Here we describe extendable linear, curved and angled protein building blocks, as well as inter-block interactions, that conform to specified geometric standards; assemblies designed using these blocks inherit their extendability and regular interaction surfaces, enabling them to be expanded or contracted by varying the number of modules, and reinforced with secondary struts. We construct twistless helix repeat (THR) protein blocks from identical straight α-helices (typically 2–4 helices in each unit); the length of the blocks can be varied simply by varying the number of repeat units. Restricting helical geometry to ideal straight helices with zero helical twist in principle considerably limits what types of structure could be built, but this is more than compensated by the great simplification of downstream material design, as illustrated below. Using X-ray crystallography and electron microscopy, we validate nanomaterial designs ranging from simple polygonal and circular oligomers that can be concentrically nested, up to large polyhedral nanocages and unbounded straight ‘train track’ assemblies with reconfigurable sizes and geometries that can be readily blueprinted.

To generate expandable nanocages, flat cyclic components that form the faces of the cages were linked through noncovalent handshake interactions at the specified angle. For the flat cyclic component, we used a ring design with 12 repeats (R12B) constructed from curve units, and split the 12 repeats into either 3 subunits with 4 repeats each (C3) or 4 subunits with 3 repeats each (C4), depending on the desired polyhedral symmetry architecture. We then fused linear THR arms onto each subunit constrained to point outward parallel to a radial vector emanating from the symmetry axis, but offset such that when the C2 interface is formed, the C2 axis is along a radial vector. For tetrahedra (T3), octahedra (O3) and icosahedra (I3) built from flat C3-symmetric objects, the out-of-plane handshake angles that are needed to join the flat objects are 70.5°, 109.5° and 138.2°, respectively. Tetrahedral, octahedral ‘cubic’ and icosahedral structures with C3 rings at respective axes (T3, O3 and I3), and octahedral structures with C4 rings at the respective axes (O4) were constructed by incorporation of the appropriate C2 interface. Designed geometric features including the spindle-like twofold handshake interface and the flat ‘in-plane’ ring areas with distinct holes are clearly evident.

>MEELREIAERAEADMREISELAEELVEDPVYAVAVRGMALVGAAGVFALGVGGPPEVLEEARRRVEEAAREALRKYEEGADVSELVAELIRETSRQIAEIAEATIKATDDPEVLEEISEFAEERSRRLSEYAERHVTNPILAATVVALAEVLSAVVRARSYGAPEEVGEKAVKEVREASEEALERYKKGEDVSELVAELIRETSRQIAEIAEATIKATDDPEVLEEISEFAEERSRRLSEYAERHVTNPILAATVVALAEVLSAVVRARSYGAPEEVGEKAVKEVREASEEALERYKEGADESELVAEVMTATAEAVGEIAEATIEATDDPEKRRKIAEFAREKMRRIRELARKLVEDPVLAAAVAARALVLSAAVFAKAYGGPEEYSRLMRRWVEKAAELARRARRLGADESVLVAALMRVAAIAVTAIAMMTVMGVQNAPPEERERILAEATEMIARVLAEATRRVMKRLEDPEAAAELALATIEAITELFVDALEIIRSGEVASRLAKSGIEVIAELAEAAIEHIDDPEQLKKIVKKAAEAIKKIVEELIKKDVEDELLAEVTSEGNRKLSRITSKALTKIKDEKAAAELTIEAIEAITENFLLALERIKDGEVAAKLAEDGLLEIYRLAVSGIEHIDNPEELEKIVKKTEEAVERIVEALEKKDVEPELKEEVEELGKKLVEIVRKLAERKGGSGGSWGHHHHHHG[12x]> AFMPDARAYWVTSDLIAWNVGELEAQSVCLYASRAAAMSLSPSNGGIQGYDSKVELQPESAGLPETVTQKFPFISSYRAFRVPSSVDVASLVKCQLVVASFGADGKHVDVTGLQLPGVLDDMFAYTGPLGAVFSEDSVSLHLWAPTAQGVSVCFFDGPAGPALETVQLKESNGVWSVTGPREWENRYYLYEVDVYHPTKAQVLKCLAGDPYARSLSANGARTWLVDINNETLKPASWDELADEKPKLDSFSDITIYELHIRDFSAHDGTVDSDSRGGFRAFAYQASAGMEHLRKLSDAGLTHVHLLPSFHFAGVDDIKSNWKFVDECELATFPPGSDMQQAAVVAIQEEDPYNWGYNPVLWGVPKGSYASDPDGPSRIIEYRQMVQALNRIGLRVVMDVVYNHLDSSGPCGISSVLDKIVPGYYVRRDTNGQIENSAAMNNTASEHFMVDRLIVDDLLNWAVNYKVDGFRFDLMGHIMKRTMMRAKSALQSLTTDAHGVDGSKIYLYGEGWDFAEVARNQRGINGSQLNMSGTGIGSFNDRIRDAINGGNPFGNPLQQ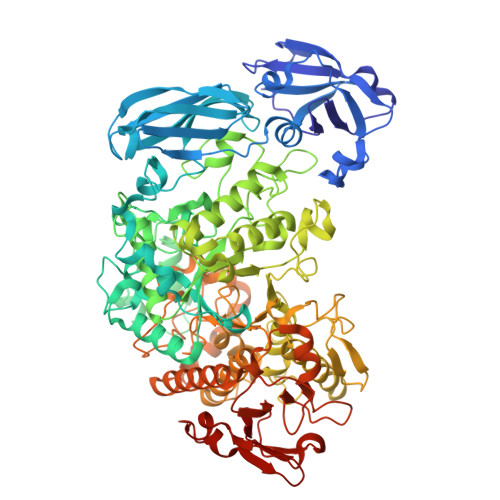GFNTGLFLEPNGFYQGNEADTRRSLATYADQIQIGLAGNLRDYVLISHTGEAKKGSEIHTFDGLPVGYTASPIETINYVSAHDNETLFDVISVKTPMILSVDERCRINHLASSMMALSQGIPFFHAGDEILRSKSIDRDSYNSGDWFNKLDFTYETNNWGVGLPPSEKNEDNWPLMKPRLENPSFKPAKGHILAALDSFVDILKIRYSSPLFRLSTANDIKQRVRFHNTGPSLVPGVIVMGIEDARGESPEMAQLDTNFSYVVTVFNVCPHEVSMDIPALASMGFELHPVQVNSSDTLVRKSAYEAATGRFTVPGRTVSVFVEPRC> MLDRLDAALRFQQEALNLRAQRQEILAANIANADTPGYQARDIDFASELKKVMVRGREETGGVALTLTSSHHIPAQAVSSPAVDLLYRVPDQPSLDGNTVDMDRERTQFADNSLKYQMGLTVLGSQ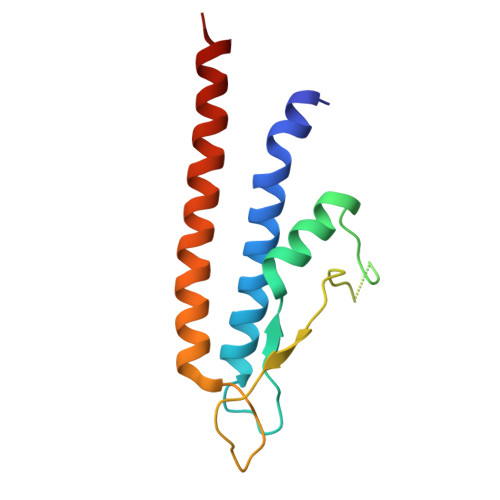LKGMMNVLQGGN4-[(3-aminophenyl)amino]pyrido[2,3-d]pyrimidin-5(8H)-one 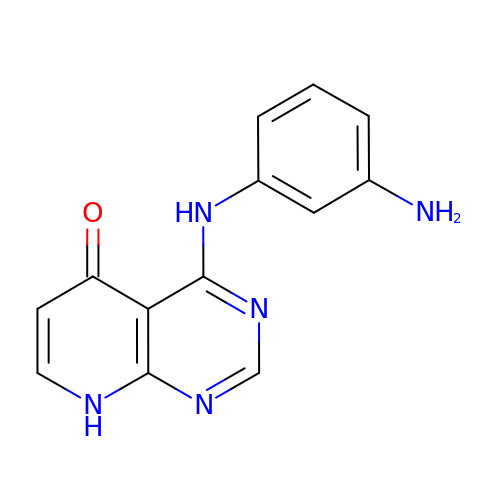| C13 H11 N5 O | ZHTCGJQGXHCVHH-UHFFFAOYSA-N> GSHMSKKILIVESDTALSATLRSALEGRGFTVDETTDGKGSVEQIRRDRPDLVVLAVDLSAGQNGYLICGKLKKDDDL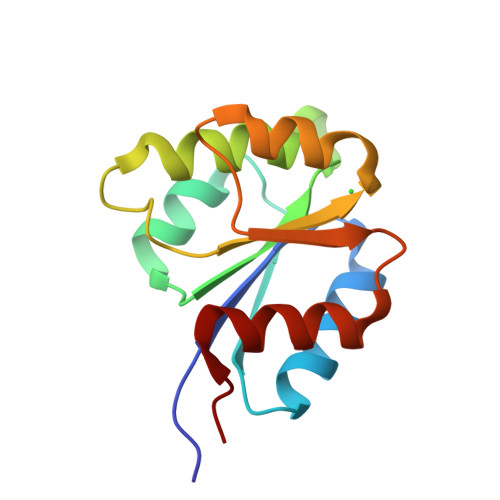KNVPIVIIGNPDGFAQFRKLKAHADEYVAKPVDADQLVERAGALIGFPE>MDEGELMRLMKRRILESYRWQEDVVKPLSRELEIDVEEFQDILMDKLDMSSLEALHPRFESARPRCIREKLHSDLQLCWLVDVMEIISVDDAEALKDE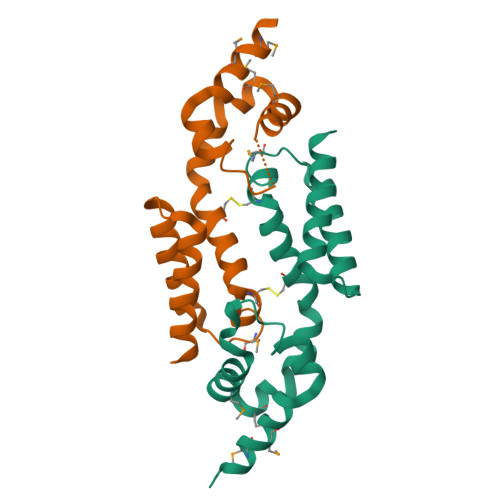ITELVLAGREYSEALSEGRRRLHEILRS[2x]> ENLYFQGMTFEHIISSKRLEGFLRHLAEEGVGGVEPLAKGTTSLVFTGVLGGRKVVIKLQRPDSPRSNFEKEAELTKIASTFGVTPPIIGLGEFEGLPYLIREFAEGEPILFADVEKEHLFRIVEKTALLDRLGIDHGQIQGGKHIIIGEDVYLIDFEKAGFRKPNNLTSAMAMIFIGENAISKRVREKFGLDEKFREEMKDALRHYKRTGSLSRLLSLLSGL

Here we identified 2′-phosphouridine (Up) at position 47 of tRNAs from thermophilic archaea. Up47 confers thermal stability and nuclease resistance to tRNAs. In addition, we identified the arkI gene, which encodes an archaeal RNA kinase responsible for Up47 formation. Taken together, our findings show that Up47 is a reversible RNA modification mediated by ArkI and KptA that fine-tunes the structural rigidity of tRNAs under extreme environmental conditions.

To find the structural basis of Up47 formation, we crystallized TkArkI and determined its atomic structure at a resolution of 1.8 Å using X-ray crystallography. As observed for ePKs, TkArkI also consisted of two lobes, termed the N-terminal and C-terminal lobes, which were connected by a hinge (positions 96–109). ePKs consist of 12 conserved subdomains that fold into the catalytic core. TkArkI had subdomains I–V in the N-terminal lobe and subdomains VIab, VII, IX and XI in the C-terminal lobe, but lacked subdomains VIII and X. The HRD triplet in the catalytic loop (VIb) of ePKs was replaced with HGQ in TkArkI. In addition, the DFG triplet in the metal-binding loop (VII) of ePKs was replaced with DFE in TkArkI. Although we demonstrated that TkArkI is an ATP-dependent RNA kinase involved in the formation of Up47, we observed a clear electron density for guanosine in the cleft of the two lobes, which corresponds to the ATP-binding site of ePKs surrounded by the hinge and metal-binding, catalytic and P-loops. However, in the guanosine-bound TkArkI structure, the P-loop was dislocated from the ligand-binding site. In homology modelling to ePKs, ATP virtually bound to the active form of the ligand-binding site of TkArkI. It is likely that the P-loop and other motifs form the active pocket for ATP binding following tRNA binding to TkArkI. The electrostatic surface potential showed a large positive area on one side of the TkArkI structure. Instead of the missing subdomain VIII involved in recognition of substrate peptide in ePKs (mouse PRKACA), the basic surface in the C-terminal lobe might bind substrate tRNA through electrostatic interaction.> GPGSEFSLDHSDLVAELLKELSNHNERVEERKIALYELMKLTQEESFSVWDEHFKTILLLLLETLGDKEPTIRALALKVLREILRHQPARFKNYAELTVMKTLEAHKDPH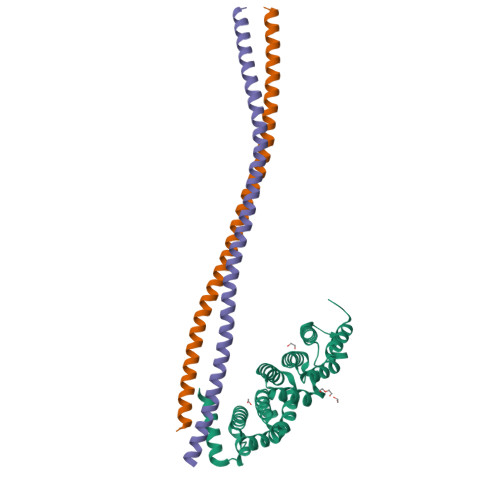KEVVRSAEEAASVLATSISPEQCIKVLCPIIQTADYPINLAAIKMQTKVIERVSKETLNLLLPEIMPGLIQGYDNSESSVRKACVFCLVAVHAVIGDELKPHLSQLTGSKMKLLNLYIKRAQTGS;>[2x]GPGSTTALQEALKEKQQHIEQLLAERDLERAEVAKATSHVGEIEQELALARDGHDQHVLELEAKMDQLRTMVEAADREKVELLNQLEEEKRKVEDLQFRVEEESITKGDLE Glycosylation catalyzed by a series of glycosyltransferases is crucial for biogenesis of SRRP adhesins in Gram-positive bacteria. dGT1 is a unique bifunctional protein involved in the biosynthesis of an SRRP adhesin Fap1 of S. parasanguinis. It is essential for glycosylation of Fap1 by two distinct glycosyltransferase activities derived from the N-terminal and C-terminal regions, respectively. In this study we demonstrate that the C terminus of dGT1 (CgT) is an independent glycosyltransferase, transferring GlcNAc to the Glc-Glc-GlcNAc-modified Fap1. Thus we conclude that CgT catalyzes the fourth step of Fap1 following the action of Gtf1/Gtf2, Gtf3, and DUF1792.

The x-ray crystal structure of CgT (286–582 amino acids) was determined at 2.4-Å resolution. The space group of the CgT structure is R3, shown in dimer in symmetry unit. Each CgT monomer has a triangle shape and contains three regions: an N-terminal domain, a core region, and a helix domain. The N-terminal region consists of β1-β2-β3-β4 and α1-α2-α3. β1, β2, and β3 make a parallel β-sheet surrounded by α1, α2, and α3 to form a Rossmann-fold. The core region consists of six strands (β5 to β10) and six helixes (α4 to α9). β7, β8, β9, and β10 lined in the center clamped by α5, α6, and α7 form a sandwich shape. At the very C terminus there is a unique helix domain consisting of three helices. In the CgT structure, two monomers bind tail to tail together through the helix domain. Because all key binding residues of this CgT dimer were located in the helix domain, we designate it as a helical binding domain. CgT contains a unique helix binding domain in addition to possessing a typical GT-A-type glycosyltransferase domain. Noticeably, this helix arm is not crucial for GlmU activities. This is in sharp contrast to the helix domain of CgT, which is important for enzymatic activity of CgT in addition to its role in the oligomerization of dGT1.

>MDNGELISIIVPVYNVEKYLKRCLDSLLRQTYKNFEIILINDGSTDNSSIICEEYAKIDNRIQILHQTNAGPSAARNAGITYASGKYITFVDSDDFVEEFYLEHLYRALVDNGSDISVCNFNSFNEDRQSFLFSITKEKYFCKNYTIAEWMDLESSANNNLFLTFTFSPTKLFKAELFEGIRFPLGRLREDDATIYRLYLKASQITFINEGSYYYSQRSEGLSRTRMLDDISSMISNAEERIALLASMGYDLTEQIKSYKGRLKKCCEDALRNGQIELYQQCCNKLDLIENYPKEK[2x]3-[(1-methyl-6-oxidanylidene-pyridin-3-yl)carbonylamino]benzoic 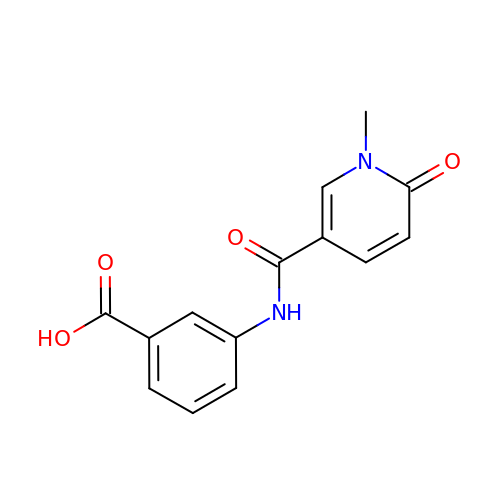acid | C14 H12 N2 O4 | BLNCOMMFECMGRC-UHFFFAOYSA-N> MQYDDDWQYEDCKLARGGPPATIVA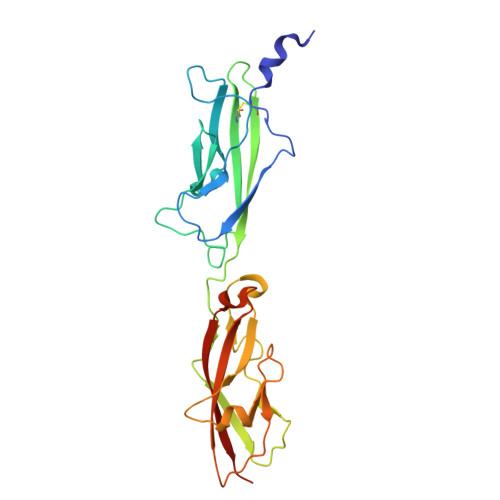IDEESRNGTILVDNMLIKGTAGGPDPTIELSLKDNVDYWVLLDPVKQMLFLNSTGRVLDRDPPMNIHSIVVQVQCVNKKVGTVIYHEVRIVVRDRNDNSPTFKHESYYATVNELTPVGTTIFTGFSGDNGATDIDDGPNGQIEYVIQYNPEDPTSNDTFEIPLMLTGNVVLRKRLNYEDKTRYYVIIQANDRAQNLNERRTTTTTLTVDLEHHHHHH>[2x]MSDTLPGTTPPDDNHDRPWWGLPCTVTPCFGARLVQEGNRLHYLADRAGIRGRFSDVDAYHLDQAFPLLMKQLELMLTGGELNPRHQHTVTLYAKGLTCEA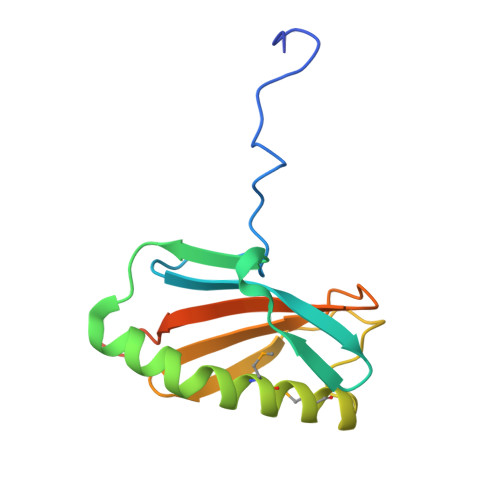DTLGSCGYVYLAVYPTPAAPATTVLEHHHHHH>[3x]MPSVYGARLTTFEDEEKESEYGYVRKVSGPVVIADGMNGAAMYELVRVGHDNLIGEIIRLEGDSATIQVYEETAGLMVNDPVLRTHKPLSVELGPGILGNIFDGIQRPLKTIAIRSGDVYIPRGVSVPALDKDTLWEFQPKKIGEGDLLTGGDLYATVFENSLMQHHVALPPDAMGKVTYVAPAGQYSLKDTVLELEFQGVKKSFTMLQAWPVRTPRPVSSKLAADTPLLTGQRVLDALFPSVLGGTCAIPGAFGCGKTVISQALSKYSNSDTVVYVGCGERGNEMAEVLMDFPQLTMTLPDGREESVMKRTTLVANTSNMPVAAREASIYTGITIAEYFRDMGYNVSMMADSTSRWAEALREISGRLAEMPADSGYPAYLAARLASFYERAGKVKCLGGPERTGSVTIVGAVSPPGGDFSDPVTSATLSIVQVFWGLDKKLAQRKHFPSVNWLISYSKYSTALESFYEQFDPDFINIRTKAREVLQREDDLNEIVQLVGKDALAEGDKITLETAKLLREDYLAQNAFTPYDKFCPFYKSVWMMRNIIHFYNLANQAVEKGAGMDGQKITYTLIKHRLGDLFYRLVSQKFEDPAEGEPALVAKFKKLHEDLTAGFRALED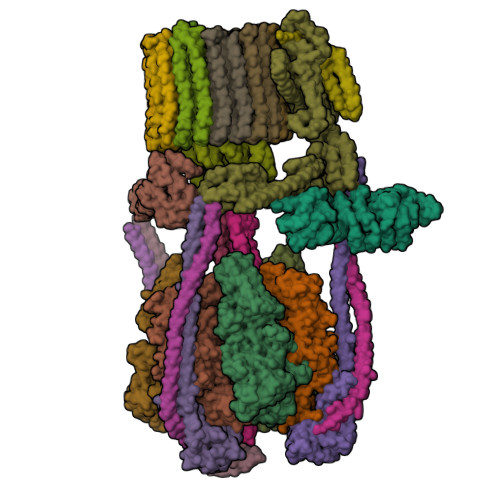ETR;>[3x]MGVAQNNVDMEEGTLEVAMEYRTVTGVAGPLVILDKVKGPKYYEIVNIRLGDGTMRRGQVLEVDGEKAVVQVFEGTSGIDNKFTTVQFTGEVLKTPVSLDMLGRIFNGSGKPIDNGPPILPEAYLDISGSSINPSERTYPEEMIQTGISTIDVMNSIARGQKIPLFSAAGLPHNEIAAQICRQAGLVKRLEKTDNLLEDGEEDNFAIVFAAMGVNMETAQFFKRDFEENGSMERVTLFLNLANDPTIERIITPRIALTTAEYLAYECGKHVLVILTDMSSYADALREVSAAREEVPGRRGYPGYMYTDLAQIYERAGRIEGRKGSITQIPILTMPNDDITHPTPDLTGYITEGQIYIDRQLQNRQIYPPINVLPSLSRLMKSAIGEGMTRRDHSDVSNQLYANYAIGKDVQAMKAVVGEEALSSEDLLYLEFLDKFERKFVAQGAYDSRNIFQSLDLAWTLLRIFPRELLHRIPGKTLDQYYSRDAAN;>[3x]MNDADVSKQIQQMVRFIRQEAEEKANEISVSAEEEFNIEKLQLVEAEKKKIRQEYERKEKQVEIRKKIEYSMQLNASRIKVLQAQDDLVSNMMEAASKEVLNVSRDHNSYKKLLKGLIVQSLLRLKEPAVLLRCRKDDHHLVESVLESAKEEYAQKLQVHPPEIIVDHHIYLPPGPGHHNAHGPSCSGGVVVASRDGKIVCENTLDARLDVVFRKKLPEIRKQLVSQVAA;>[3x]MASNRGHGGIQQLLAAEQEAQHIVAAARNAKMARLRQAKEEAEREIAEHRAQVEREFQRKLAESSGDSGANVKRLEQETEVKIHHLNAGAEKIQYDVVQMLLKHVTTVKN;> MAQNQRLTVVPTVTMLGVMKSRLVGATRGHALLKKKSDALTVQFRQILKNIVTTKESMGEVMKDSSFALIEAKYVAGENIKHIVLENVQNASIKVRSRQENIAGVKIPKFEYFTDGETKNDLTGLARGGQQVQQCRAAYVKAIELLVELASLQTSFLTLDEAIKTTNRRVNALENVVKPRLENTITYIKGELDELEREDFFRLKKIQGYKKREIERQLASSKQFVEEQFAEKVSLQKGISIKSAQNLLSAGEKDEDIIF;> MAGRAQIPTKSSALIAMIADEDTVTGFLLAGVGNVDLRRKTNYLIVDSKTTVKAIEDAFKEFTTKEDIAIVLISQYVANMIRFLVDSYNKPIPAILEIPSKDHPYDPAHDSVLSRVKNLFSAESVASGRR;> MASRYWVVSLPVQNSAASVWNRLQEQISKHSFDTPLYRFNIPNLRVGTLDSLLALSDDLVKSNSFVESVSHKIRRQIEELERVSGIESSSLSVDGVPVDTYLTRFVWDEAKYPTMSPLREIVDGIHTLVAKIEDDLKVRVAEYNNVRSQLNAINRKQSGSLAVRDLSNLVKPEDIITSEHLVTLLAVVPKYSQKDWLASYETLTSYVVPRSSKLLYEDNEYALYTVTLFGRVADNFRIAAREKGFQIRDFEYSSEAQESRNQELEKLVHDQESLRSSLLQWCYTSYGEVFSSWMHFCAVRVFAESILRYGLPPSFLACVLAPSVKGEKKVRSILEELCGNANSTFWKSEDDGGMMAGLGGDADSHPYVSFTINLV;> MDHAELTTEQVLKRDIPWETYMTTKLISGTGLQLLRRYDNRSESHRAQLLDDDGPSYVRVFVSILRDIYKEETVEYVLALIDEMLTANPKRARLFHDKSLASEDTYEPFLRLLWKGNWFIQEKSCKILASIVSARPKPQDRFFANGEASNSKSKSTTIDDVLKLLVEWLCAQLKKPSHPSRGVPVAINCLAALLKEPMVRSSFVQADGVKLLTPLISPASTQQSIQLLYETCLCVWLLSYYEPAVEYLATTRTLPRLIDVVKSSTKEKVVRVVVLILRNLLPKGNFAAQMIDLGLPQVVQSLKAQAWSDEDLLEGLNQLEEGLKDNIKRLSSFDKYKQEVLLGHLDWSPMHKDPLFWRDNITNFEENDFQILRVLLTILDTSSDPRALAVACFDLSQFIQYHPAGRVIVTDLKAKERVMKLMNHENTEVTKSALLCIQRLFLGAKYASFLQA;> MAELQSGGGGGCCPPMDLFRSEPMQLVQIIIPIESAHLTVSYLGELGLLQFKDLNSEKSPFQRTYAAQIKKCAEMARKLRFFKEQMLKAGILSSVKSTTRADNNTDDLEVKLGDLEAELVEINANGDKLQRAHSELVEYKLVLQKAGEFFSSALTSAAAQQREMESQQTGEMTIETPLLTDKEMSADPSKQIKLGFIAGLVPREKSMSFERMLFRATRGNVFLRQAVVDEPVVDPVSGEKMEKNVFVVFYSGERAKNKILKICDAFGANRYPFNEEFDKQAQAISEVSGRLSELKTTLDAGLLHRGNLLQTIGDQFEQWNLLVKREKSIYHTLNMLSLDVTKKCLVGEGWSPVFATKQIQDALERAAFDSNSQVGAIFQVLHTKESPPTYFRTNKFTSAFQEIVDAYGVAKYREANPGVFTIVTFPFLFAVMFGDWGHGICLLLGTLVLIVREKKLASQKLDDITDMTFGGRYVILMMALFSIYTGLIYNEFFSVPFEIFSHSAYACRDLSCSEATTVGLIKVRDTYPFGVDPVWHGSRSELPFLNSLKMKMSILLGVAQMNLGIILSYFNATFFRIGVNIWCQFIPQIIFLNSLFGYLSLLIILKWITGSQADLYHVMIYMFLSPTDELGDNQLFPGQKTAQLVLLLLAFVSVPWMLLPKPFILKMQHQDRHQGQSYEALQSTDESLQPDTNHDSHGHEEFEFSEVFVHQMIHTIEFVLGAVSNTASYLRLWALSLAHSELSSVFYEKVLLLAWGYNNILILIVGIIVFIFATVGVLLVMETLSAFLHALRLHWVEFQNKFYEGDGYKFSPFSFALLDDEDE;> MSGSVMLGESSSWSRALVKISPYTFSAIGIAVAIGVSVLGAAWGIYITGSSLIGAAIKAPRITSKNLISVIFCEAVAIYGVIVAIILQTKLESVPASQIYAPESLRAGYAIFASGIIVGFANLVCGLCVGIIGSSCALSDAQNSSLFVKILVIEIFGSALGLFGVIVGIIMSAQASWPAKPV;> MYGFEAMTFNIHGGYLEAIVRGYRAGLLTAADYNNLCQCETLDDIKMHLSATEYGPYLQNEPSPLHTTTIVEKCTLKLVDEYKHMLCQATEPLSTFLEYITYGHMIDNVVLIVTGTLHERDVQELLEKCHPLGMFDSIATLAVAQNMRELYRLVLVDTPLAPYFSECITSEDLDDMNIEIMRNTLYKAYLEDFYKFCQKLGGATAEIMSDLLAFEADRRAVNITINSIGTELTRDDRRKLYSNFGLLYPYGHEELAVCEDIDQVRGVMEKYPPYQSIFSKLSYGESQMLDKAFYEEEVKRLCLAFEQQFHYGVFFAYMRLREQEIRNLMWISECVAQNQKSRVHDSVVFIF;> MGFLVTTLVFLVIGIIASLCTRICCNRGPSTNLLHLTLVITATVSCWMMWAIVYLAQMKPLIVPILSEEE;>MSTFSGDETAPFFGFLGAAAALVFSCMGAAYGTAKSGVGVASMGVMRPELVMKSIVPVVMAGVLGIYGLIIAVIISTGINPKAKSYYLFDGYAHLSSGLACGLAGLSAGMAIGIVGDAGVRANAQQPKLFVGMILILIFAEALALYGLIVGIILSSRAGQSRAE[9x]URIDINE-DIPHOSPHATE-METHYLENE-N-ACETYL-GLUCOSAMINE | C18 H29 N3 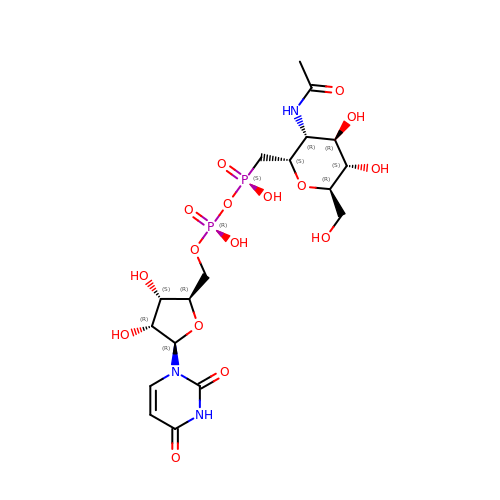O16 P2 | KUFKOJZYUNOEES-DLLWPQOWSA-N>GKINDWEEPRLDIEGFVVDYFTHRIRQNGMEWFGAPGLPCGVQPEHEMMRVMGTIFEKKHAENFETFCEQLLAVPRISFSPYQDVVRTVGNAQTDQCPMSYGRLIGLISFGGFVAAKMMESVELQGQVRNLFVYTSLFIKTRIRNNWKEHNRSWDDFMTLGKQMKEDYER[2x];>DSSQFADDSGFFDDSEISSIGYEIGSKLAAMCDDFDAQMMSYSAHASDRSLFHRLLD[2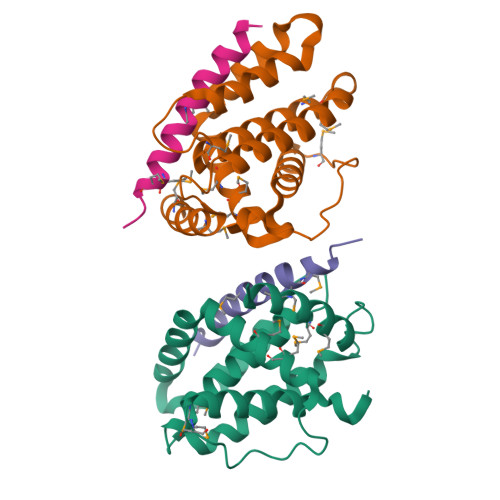x]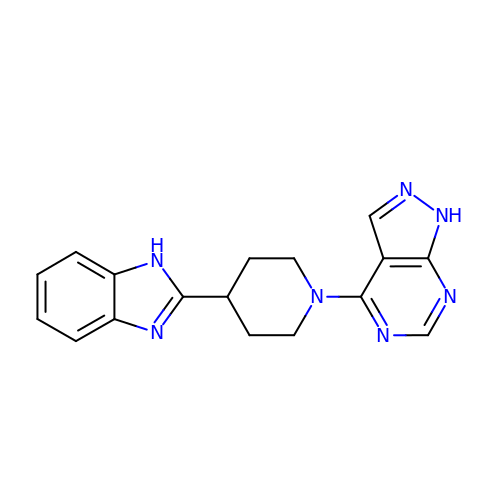4-[4-(1H-benzimidazol-2-yl)piperidin-1-yl]-1H-pyrazolo[3,4-d]pyrimidine | C17 H17 N7 | SAOVCWDCHHZCCL-UHFFFAOYSA-N>[4x]MTLLSPGIELKETTVQSTVVNNSTGTAALAGKFQWGPAFQIKQVTNEVDLVNTFGQPTAETADYFMSAMNFLQYGNDLRVVRAVDRDTAKNSSPIAGNIEYTISTPGSNYAVGDKITVKYVSDDIETEGKITEVDADGKIKKINIPTAKIIAKAKEVGEYPTLGSNWTAEISSS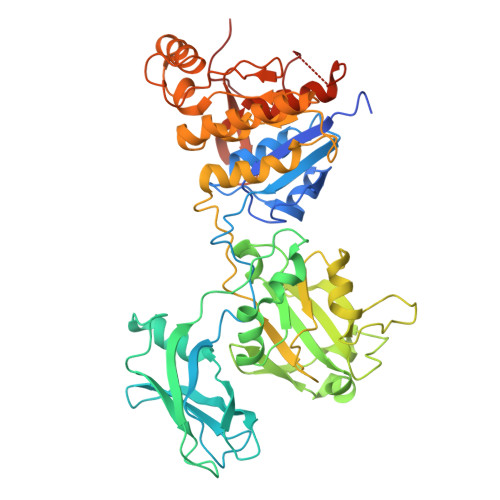SSGLAAVITLGKIITDSGILLAEIENAEAAMTAVDFQANLKKYGIPGVVALYPGELGDKIEIEIVSKADYAKGASALLPIYPGGGTRASTAKAVFGYGPQTDSQYAIIVRRNDAIVQSVVLSTKRGGKDIYDSNIYIDDFFAKGGSEYIFATAQNWPEGFSGILTLSGGLSSNAEVTAGDLMEAWDFFADRESVDVQLFIAGSCAGESLETASTVQKHVVSIGDVRQDCLVLCSPPRETVVGIPVTRAVDNLVNWRTAAGSYTDNNFNISSTYAAIDGNYKYQYDKYNDVNRWVPLAADIAGLCARTDNVSQTWMSPAGYNRGQILNVIKLAIETP>MGSSHHHHHHSSGLVPRGSHMASATKNASSATPATMTSMVSQRQDLFMTDPLSPGSMFFLPNGAKIFNKLIEFMKLQQKFKFGFNEVVTPLIYKKTLWEKSGHWENYADDMFKVETTDEEKEEYGLKPMNCPGHCLIFGKKDRSYNELPLRFSDFSPLHRNEASGALSGLTRLRKFHQDDGHIFCTPSQVKSEIFNSLKLIDIVYNKIFPFVKGGSGAESNYFINFSTRPDHFIGDLKVWNHAEQVLKEILEESGKPWKLNPGDGAFYGPKLDIMVTDHLRKTHQVATIQLDFQLPERFDLKFKDQDNSYKRPIMIHRATFGSIERFMALLIDSNEGRWPFWLNPYQAVIIPVNTKNVQQLDMCTALQKKLRNELEADDMEPVPLNDWHFNVDLDIRN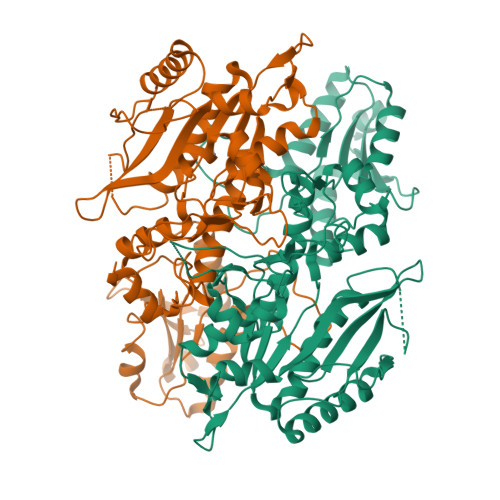EPVGYRIKSAILKNYSYLIIVGDEEVQLQKYNIRERDNRKSFEKLTMSQIWEKFIELEKNYK[4x]>[2x]TNMSIKEQRESLPVFQFRDQIIQAVKDNQILIVVGETGSGKTTQVTQYLAEAGFTKYGMIGCTQPRRVAAVSVAKRVAEEVGCQLGQEVGYTIRFEDVTSPATKIKYMTDGMLQREILMDPDLKRYSVIMLDEAHERTIATDVLFALLKKTVKRRPDLKVIVTSATLDAEKFSEYFNSCPIFTIPGRTFPVEILYSREPEPDYLEAALTTVMQIHLTEPPGDILVFLTGQEEIDTACEILYERMKALGPSVPELIILPIYSALPSEMQSRIFEPAPPGSRKVVIATNIAETSITIDYIYYVVDPGFVKQNAYDPKLGMDSLVVTPISQAQANQRAGRAGRTGPGKCFRLYTEAAYQSEMLPTTIPDIQRQNLANTILLLKAMGINDLLRFDFMDPPPVNTMLTALEELYALGALDDEGLLTRLGRKMADFPMEPSLSKVLIASVDKGCSDEMVTIVSMLNLQQIFYRPKDKQQQADQKKAKFHDPTGDHLTLLNVYNAWKNSGYSNAWCFENYIQARAMRRARDVRQQIVKIMERHRHPIISCGRDTDKIRQALCAGFFRNTARKDPQEGYKTLTEGTPVYLHPSSALFGKQAEWVLYHELVLTTKEYMHFTTAIEPKWLVEAAPTFFKLAPTDRLSKRKKAERIQPLYNKYEGEDGWRLSAQRRAARPGGGGGTWG

DEAH-box adenosine triphosphatases (ATPases) play a crucial role in the spliceosome-mediated excision of pre-mRNA introns. The catalytic activation, the catalysis itself as well as the final disassembly steps are driven by so-called DEAH-box helicases. They all belong to the helicase superfamily 2 (SF2) and share at least eight conserved sequence motifs (motifs I, Ia, Ib, II, III, IV, V and VI) spread over two RecA-like domains that together form the helicase core. Two RecA-like domains, referred to as RecA1 and RecA2, build up the helicase core. The RecA2 domain contains an anti-parallel β-hairpin present in all DExH-box helicases, which protrudes out of the RecA2 domain thereby contacting the C-terminal domains. These domains are divided in three distinct domains, namely the winged-helix (WH), the helix-bundle (HB) and the oligonucleotide-binding (OB) domain.

An additional crystal structure of Prp22 in absence of RNA and adenosine nucleotide could be solved. The two Prp22 molecules found in the asymmetric unit exhibit virtually identical organization of the RecA1 and C-terminal domains, but strongly differ in the position of the RecA2 domain with respect to rest of the protein. Although significantly elevated B-factors of the RecA2 domain did not allow to build a complete model of this domain (133 of 173 RecA2 residues for Apo1 and 141 of 173 RecA2 residues for Apo2), enough portions of the domain were traceable in the electron density to unambiguously place it with respect to the RecA1 and C-terminal domains. The two different positions of the RecA2 domain together with the increased B-factor values suggest that in absence of any interaction partner this domain has a high degree of freedom to move as a rigid body. In contrast to previously solved adenosine nucleotide-bound structures of genuine DEAH-box ATPases, the RecA2 domains of both Apo structures display an increased distance toward the RecA1 domain. While the RecA1-RecA2 center of mass distance ranges between 27.3–27.7 Å when ADP/ATP is bound, this distance is increased to up to 31 Å in the unliganded state. The intrinsic mobility of the RecA2 domain allows the helicase core to adopt more open conformations than were previously known from adenosine nucleotide-bound structures. A Prp22 Apo structure highlights the mobility of the RecA2 domain in the absence of any adenosine nucleotide. After the release of the ADP, all nucleotide-mediated interactions between both RecA-like domains are lost. Together with the loss of contact of the RecA2 domain with the RNA backbone, this probably enables a complete detachment of the RecA2 domain and allows independent movement as implied by the Prp22 Apo structure. In contrast, without bound RNA the RecA2 domain is not optimally prepositioned due to its intrinsic mobility, leading to a prolonged ATP sensing time.>[2x]MGHHHHHHHHHHSSGHIDDDKHMVNVKKEFVDNMFSVKGKVALVTGATGALGCVLSKAYGYAGAKVFMTG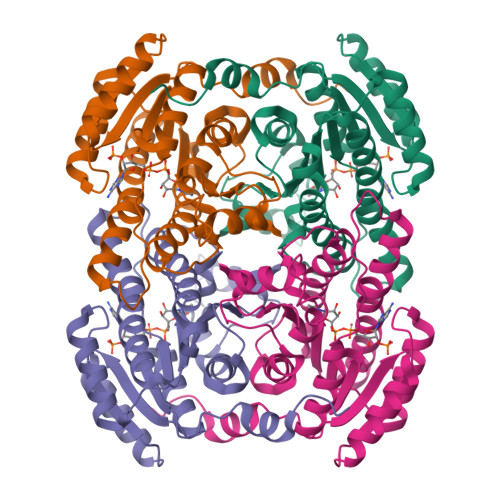RNEKKLQALEAEFKAEGIDCAYGVADPADEAQVDAMITACVAQYGEVNILAVTHGFNKPQNILEQSVADWQYIMDADCKSVYVVCKYVAQQMVDQGKGGKIVVVTSQRSKRGMAGYTGYCTSKGGADLMVSSMACDLSAKYGINVNSICPTVFRSDLTEWMFDPESAVYQNFLKREPIGRLAEPEDFVGYALFLSSDASNYITGANCDCSGGYLTC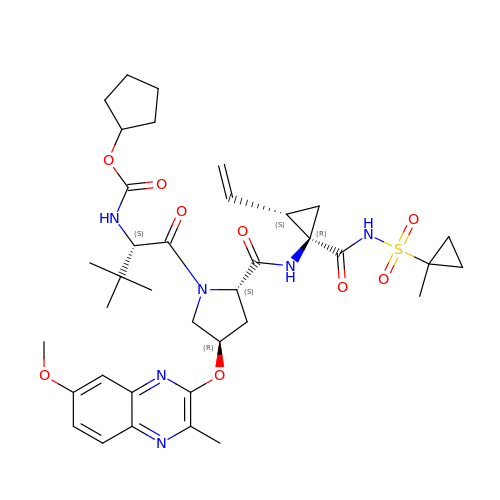N-[(cyclopentyloxy)carbonyl]-3-methyl-L-valyl-(4R)-N-[(1R,2S)-2-ethenyl-1-{[(1-methylcyclopropyl)sulfonyl]carbamoyl}cyclopropyl]-4-[(7-methoxy-3-methylquinoxalin-2-yl)oxy]-L-prolinamide | C37 H50 N6 O9 S | XMUMASNXHDVGQJ-LCWNRMNXSA-N> MFAWWGRTVYQFRYIVIGVMVALCLGGGVYGISLGNHVTQSGFYDEGSQSVAASLIGDEVYGRDRTSHVVAILTPPDDKKVTDKAWQKKVTEELDQVVKDHEDQIVGWVGWLKAPDTTDPTVSAMKTQDLRHTFISIPLQGDDDDEILKNYQVVEPELQQVNGGDIRLAGLNPLASELTGTIGEDQKRAEVAAIPLVAVVLFFVFGTVIAAALPAIIGGLAIAGALGIMRLVAEFTPVHFFAQPVVTLIGLGIAIDYGLFIVSRFREEIAEGYDTEAAVRRTVMTSGRTVVFSAVIIVASSVPLLLFPQGFLKSITYAIIASVMLAAILSITVLAAALAILGPRVDALGVTTLLKIPFLANWQFSRRIIDWFAEKTQKTKTREEVERGFWGRLVNVVMKRPIAFAAPILVVMVLLIIPLGQLSLGGISEKYLPPDNAVRQSQEQFDKLFPGFRTEPLTLVMKREDGEPITDAQIADMRAKALTVSGFTDPDNDPEKMWKERPANDSGSKDPSVRVIQNGLENRNDAAKKIDELRALQPPHGIEVFVGGTPALEQDSIHSLFDKLPLMALILIVTTTVLMFLAFGSVVLPIKAALMSALTLGSTMGILTWMFVDGHGSGLMNYTPQPLMAPMIGLIIAVIWGLSTDYEVFLVSRMVEARERGMSTAEAIRIGTATTGRLITGAALILAVVAGAFVFSDLVMMKYLAFGLLIALLLDATIIRMFLVPAVMKLLGDDCWWAPRWMKRVQEKLGLGETELPDERKRPTVRESETDQRALVGVGAPPPPPRPHDPT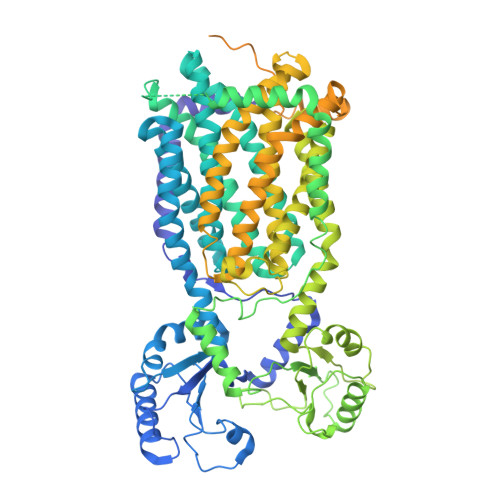HPAPEPVRPMPPMRSNAPSAAGTARISTPPQPPQPPQAPAQQAGDEPATTRFAMARNAVRNAVNSAVHGGAGSAAAPTERAPRPGGPAQPPAPPQREEREIESWLGALRGPAPAKNVPQPPAQPQRPSTDTTRAMPPQGRPPAGPADRGNENAPTTAFSAQRPPNGGAPADATTAIPTPPQREQEPSTEKLNTREDAPEDPETKRRGGGMSAQDLLRREGRLHHHHHH Human gamma-D crystallin (HGD) is a soluble, monomeric protein expressed in the eye lens during fetal development. The high expression levels contribute to the refractive index within the lens which focuses visible light upon the retina. However, this halts further expression of HGD. This means HGD must remain correctly folded and soluble for the entire human lifespan in order to maintain visual acuity. In order to observe structural changes in HGD, we take advantage of an arginine-to-serine point mutation, R36S, first identified in congenital cataracts (HGDm).

The effect of oxidation of HGDm was investigated by incubating a slurry of microcrystals at room temperature in the absence of light for nine months. After aging, DTT adduct formation is observed at 100% occupancy at C41 and C108 and oxidation at C110 to sulfenic acid. Although the fresh structure shows no significant binding of DTT, after aging of the crystals, DTT is seen to form disulfide bonds to two of the surface cysteine residues, C41 and C108 with strongly ordered density. In addition to these covalent modifications, the protein conformation is subtly different, with an overall r.m.s.d. of 0.23 Å for chain A and 0.21 Å for chain X. However, this is dwarfed by the 0.67 Å r.m.s.d. between chains A and X in the aged structure and 0.62 Å in the fresh structure. Aging of chain A leads to an expansion of the NTD and a contraction in the CTD. Aging of chain X leads to a contraction in both domains, and a notable reduction in the distance between the two. In contrast, the aged structure incurred a radiation dose of just 0.02 MGy. To control for the possibility of radiation damage-induced loss of DTT in the fresh structure, a series of 20 consecutive 5 ms exposures of each aged crystal was carried out (burst series) to accumulate a DWD of 0.31 MGy. The structure from the final timepoint showed no loss of DTT. The presence of DTT-cysteine adducts at C41 and C108 are perhaps counter-intuitive, as C110 is implicated as the major site of protein cross-linking.

>GKITLYEDRGFQGRHYECSSDHPNLQPYLSRCNSASVDSGCWMLYEQPNYSGLQYFLRRGDYADHQQWMGLSDSVRSCRLIPHSGSHRIRLYEREDYRGQMIEFTEDCSCLQDRFRFNEIHSLNVLEGSWVLYELSNYRGRQYLLMPGDYRRYQDWGATNARVGSLRRVID[2x]>[2x]GPVGYGAATTGGGNKVPVNVATFEAMQSAIDSYSGSGGLVLNYTGKFDFGTIKDVCAQWKLPAKTVQIKNKS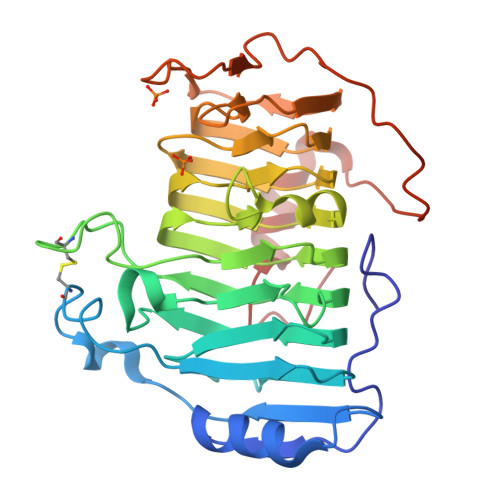DVTIKGANGSAANFGIRVVGNAHNVIIQNMTIGLLQGGEDADSISLEGNSSGEPSKIWVDHNTVFASLTKCSGAGDASFDGGIDMKKGVHHVTVSYNYVYNYQKVALNGYSDSDTKNSAARTTYHHNRFENVESRVPLQRRGLSHIYNNYFNNVTTSGINVRMGGIAKIESNYFENIKNPVTSRDSSEIGYWDLINNYVGSGITWGTPDGSKPYANATNWISTKVFPESLGYIYTVTPAAQVKAKVIATAGAGKNLAE>[3x]MAHHHHHHSSGLEVLFQGPMTHSVVELIEIESAIIQVKMQDRTHKNAFSQELTDDLIQAFEYIRQNPKYKAVILTGYDNYFASGGTQEGLLRIQQGLTAFTDDNLYSLALDCEIPVIAAMQGHGIGGGFVMGLFADIVILSRESVYTANFMKYGFTPGMGATFIVPKKLGFSLAQEILLNAGSYRGADLEKRGVPFKVLPRAEVLDYAVELAQELAEKPRNSLVTLKDHLVAPLRDQLPRVIEQELMMHEKTFHHEEVKSRIKGLYGN

In this study we present a structural and functional description of the bacillaene synthase β-branching enzymes PksH and PksI. These biocatalysts are responsible for the final two steps in β-methyl branch incorporation in this PKS/NRPS pathway. There is a single active site per PksI monomer, with each active site positioned on the periphery of the trimer, ~ 43 Å from one other. Akin to PksH, PksI adopts a characteristic CS fold, with a ββα core, that comprises two approximately perpendicular -sheets surrounded by -helices.

Assays were conducted using WT PksI, along with the point mutants PksI-H230A, PksI-H235A, PksI-K80A, PksI-K232A. Of the four PksI mutants investigated only PksI-H230A was found to be catalytically compromised, with barely detectable activity for 3-methyl glutaconyl-SNAC and significantly impaired activity for 3-methyl glutaconyl-CoA. Surprisingly, PksI-K80A and PksI-K232A both display catalytic activities akin to that of WT-PksI, with no evidence of functional impairment. In tandem with kinetic assays, the crystal structures of PksI-K80A, PksI-K232A and H230A were determined. The active sites of each of these enzymes displays the ground state “closed” conformation as observed in the WT enzyme, with no evidence of significant structural perturbations within the active site. These data thus imply that the observed kinetic effects are not attributable to global or local structural reorganization within the enzyme as a consequence of the amino acid substitutions made. Crystal structures of the mutants PksI_K80A, PksI K232A and PksI H230A revealed no significant changes in active site architecture beyond side chain identity. We thus propose a His230 dependent mechanism wherein this residue has a dual function both catalyzing decarboxylation and to act as a proton donor to the decarboxylated intermediate 7 to give the reaction product.>[4x]MAHHHHHHMSNLNGKTAVVTGAASGIGKEIALELAKAGAAVAIADLNQDGANAVADEINKAG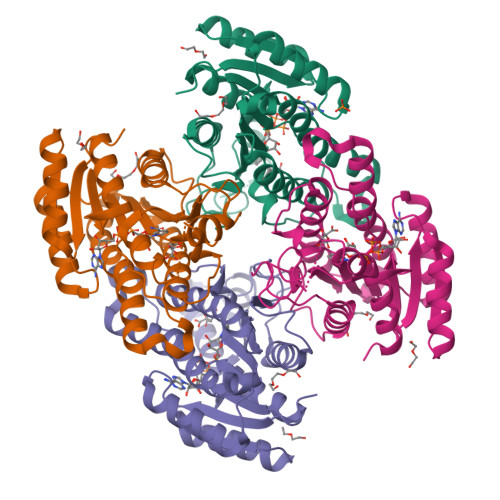GKAIGVAMDVTNEEAVNTGIDKVAEAFGSVDILVSNAGIQIVNPIENYSFADWKKMQAIHVDGAFLTTKAALKHMYKDDRGGVVIYMGSVHSHEASPLKSAYVTAKHGLLGLARVLAKEGAKHNVRSHVVCPGFVRTPLVDKQIPEQAKELGISEEEVIKKVMLGNTVDGVFTTVQDVAQTVLFLSAFPSAALTGQSFIVSHGWFMQ> MVSLDCRNTCAPAPASRLVQPPCFVCRDVFPLPVAPNPPGPVSAIIGTTPSTFSLKPDGTFITGTGISSSGSAVATDGSLELFLAPLVAHVTGSEMSPPYAVELQEGQELAIVFGATLKSGFGVRITDYYDVVFNIVSSEGTKQLKLVPGNTPSGYIWTDGEGYNIVDS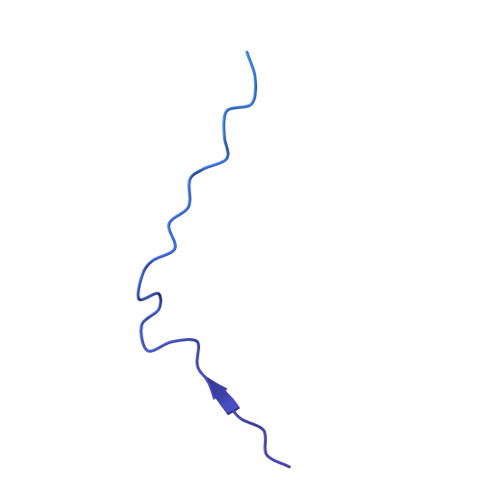NGDFHSVQNVTRPSFLGITDTGVLWQLVGYLKGTTQAELAIAIEVTVTHAN> MDRTQTFIKDCLFTKCLEDPEKPFNENRFQDTLLLLPTDGGLTSRLQRQQRKSKLNLDNLQKVSQLESADKQLEKRDYQRINKNSKIALREYINNCKKNTKKCLKLAYENKITDKEDLLHYIEEKHPTIYESLPQYVDFVPMYKELWINYIKELLNITKNL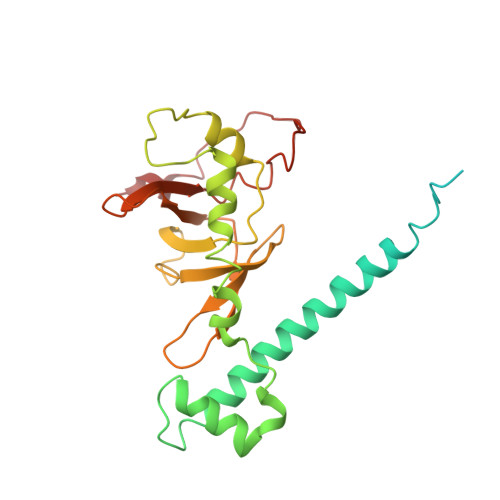KTFNGSLALLKLSMADYNGALLRVTKSKNKTLIGLQGIVIWDSQKFFIMIVKGNIIDEIKCIPKKGTVFQFEIPISDDDDSALRYSILGDRFKYRSVDRAGRKFKSRRCDDMLYYIQN3-{2-[(2',6-dimethyl[1,1'-biphenyl]-3-yl)amino]-1,3-thiazol-4-yl}propan-1-ol 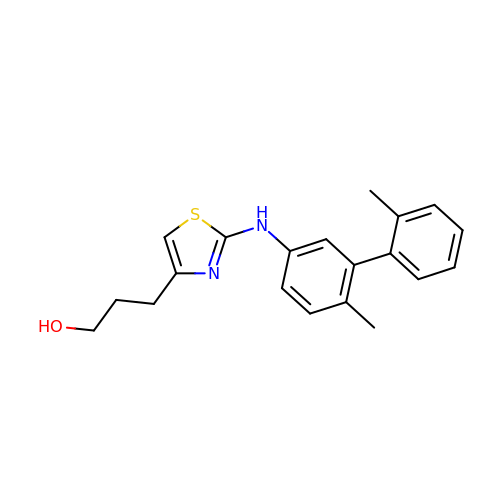| C20 H22 N2 O S | KHYLEUBWCWVZDG-UHFFFAOYSA-N>GSHMTRETERFPAREFQRDLLDWFARERRDLPWRKDRDPYKVWVSEVMLQQTRVETVIPYFEQFIDRFPTLEALADADEDEVLKAWEGL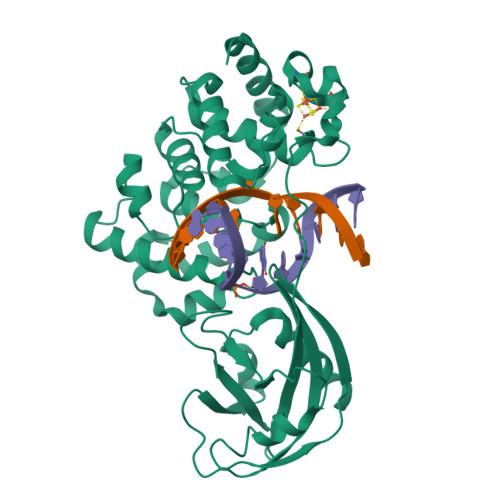GYYSRVRNLHAAVKEVKTRYGGKVPDDPDEFSRLKGVGPYTVGAVLSLAYGVPEPAVNGNVMRVLSRLFLVTDDIAKCSTRKRFEQIVREIMAYENPGAFNEALIELGALVCTPRRPSCLLCPVQAYCQAFAEGVAEELPVKMKKTAVKQVPLAVAVLADDEGRVLIRKRDSTGLLANLWEFPSCETDGADGKEKLEQMVGEQYGLQVELTEPIVSFEHAFSHLVWQLTVFPGRLVHGGPVEEPYRLAPEDELKAYAFPVSHQRVWREYKEWASGVRPPP[2x]4-hydroxy-2-oxobutanoic acid | C4 H6 O4 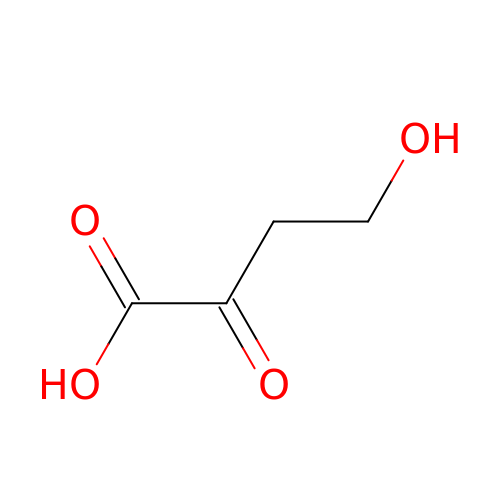| PUWWONYMIXRVQF-UHFFFAOYSA-N Citrullination, the loss of a positive charge on the arginine side chain to form citrulline, is catalyzed by peptidylarginine deiminase 4 (PAD4) of the PAD enzyme family. PAD4 is implicated in rheumatoid arthritis (RA), where citrullinated epitopes serve as important diagnostic and pathological factors. The active form of PAD4 is a homodimer, and dimerization greatly affects enzyme activity because monomeric mutants are less active. In this study, we identified GAGs as physiological allosteric coactivators of PAD4.

PAD4 activation was observed at 0.1 mM CaCl2 in our assays; therefore, we aimed to determine the PAD4–GAG complex structure under these conditions using Dp20. The obtained map showed two dimers of PAD4 connected by two Dp20 chains bound proximal to the region spanning a flexible, unresolved loop, including R123 to R137, and rich in positively charged residues (123-RTGKVKPTRAVKDQR-137). The two dimers were stacked face-to-back and angled close to 90° in the x–y plane, forming a cross-like double-propeller structure. In the x–z plane, the top dimer lies nearly flat on the bottom dimer. This organization allows interaction between the NLS region of the lower dimer (K59, K60, and K61) and the region near the Ca3-5 calcium-binding sites of the top dimer. We also determined the structure of PAD4 in the presence of Dp20 and in the absence of calcium. In this case, different structures were formed, consisting of a single PAD4 dimer with GAG oligomers spanning across the dimer to bridge two regions proximal to the N-terminal of the protein (“handbag” like structure). Importantly, these interaction anchors between the GAG and PAD4 were located near the contact surface between the monomers, encompassing the positively charged NLS. Additionally, as inferred from the density map, a GAG chain in the correct conformation can make contact with a loop containing R123. The observed change in the dimer–dimer organization between Dp12 and Dp20 at 0.1 mM Ca2+ consists of the introduction of an additional GAG anchor point for a longer Dp20 oligomer, which introduces torsion sufficient to pull the dimers together and form the 90° double-propeller, cross-like structure. This, in turn, allows for the interaction between the NLS, located in the N-terminal domain of the lower dimer, and the calcium sites Ca3-5 located on the side of the top dimer.

>MGHHHHHHHHHHHMAQGTLIRVTPEQPTHAVCVLGTLTQLDICSSAPEDCTSFSINASPGVVVDIAHGPPAKKKSTGSSTWPLDPGVEVTLTMKVASGSTGDQKVQISYYGPKTPPVKALLYLTGVEISLCADITRTGKVKPTRAVKDQRTWTWGPCGQGAILLVNCDRDNLESSAMDCEDDEVLDSEDLQDMSLMTLSTKTPKDFFTNHTLVLHVARSEMDKVRVFQATRGKLSSKCSVVLGPKWPSHYLMVPGGKHNMDFYVEALAFPDTDFPGLITLTISLLDTSNLELPEAVVFQDSVVFRVAPWIMTPNTQPPQEVYACSIFENEDFLKSVTTLAMKAKCKLTICPEEENMDDQWMQDEMEIGYIQAPHKTLPVVFDSPRNRGLKEFPIKRVMGPDFGYVTRGPQTGGISGLDSFGNLEVSPPVTVRGKEYPLGRILFGDSCYPSNDSRQMHQALQDFLSAQQVQAPVKLYSDWLSVGHVDEFLSFVPAPDRKGFRLLLASPRSCYKLFQEQQNEGHGEALLFEGIKKKKQQKIKNILSNKTLREHNSFVERCIDWNRELLKRELGLAESDIIDIPQLFKLKEFSKAEAFFPNMVNMLVLGKHLGIPKPFGPVINGRCCLEEKVCSLLEPLGLQCTFINDFFTYHIRHGEVHCGTNVRRKPFSFKWWNMVP[2x]> VVIANAHNELIHDAVLDYYGKRLATCSSDKTIKIFEVEGETHKLIDTLTGHEGPVWRVDWAHPKFGTILASCSYDGKVLIWKEENGRWSQIAVHAVHSASVNSVQWAPHEYGPLLLVASSDGKVSVVEFKENGTTSPIIIDAHAIGVNSASWAPATIEEDGEHNGTKESRKFVTGGADNLVKIWKYNSDAQTYVLESTLEGHSDWVRDVAWSPTVLLRSYLASVSQDRTCIIWTQDNEQG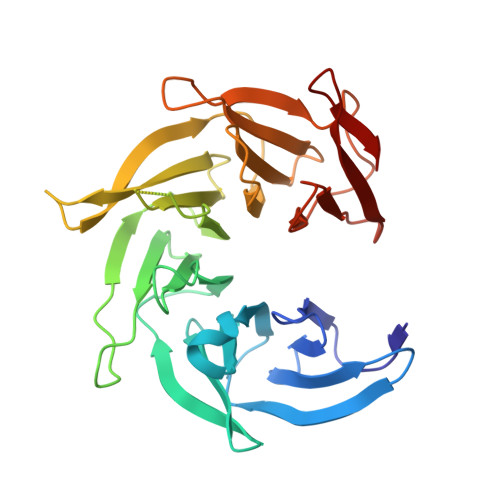PWKKTLLKEEKFPDVLWRASWSLSGNVLALSGGDNKVTLWKENLEGKWEPA> ALAPRQVLDLEDLVFTQGSHFMANKRCQLPDGSFRRQRKGYEEVHVPALKPKPFGSEEQLLPVEKLPKYAQAGFEGFKTLNRIQSKLYRAALETDENLLLCAPTGAGKTNVALMCMLREIGKHINMDGTINVDDFKIIYIAPMRSLVQEMVGSFGKRLATYGITVAELTGDHQLCKEEISATQIIVCTPEKWDIITRKGGERTYT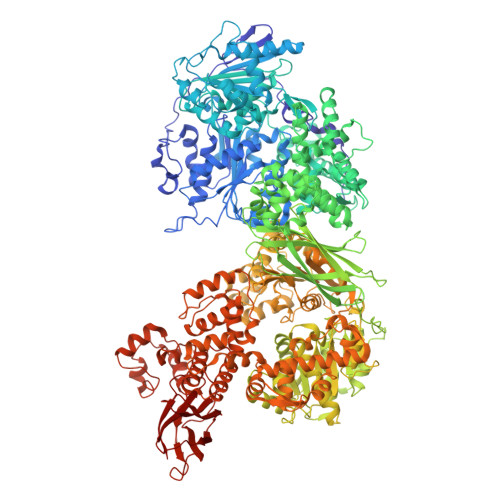QLVRLIILDEIHLLHDDRGPVLEALVARAIRNIEMTQEDVRLIGLSATLPNYEDVATFLRVDPAKGLFYFDNSFRPVPLEQTYVGITEKKAIKRFQIMNEIVYEKIMEHAGKNQVLVFVHSRKETGKTARAIRDMCLEKDTLGLFLREGSASTEVLRTEAEQCKNLELKDLLPYGFAIHHAGMTRVDRTLVEDLFADKHIQVLVSTATLAWGVNLPAHTVIIKGTQVYSPEKGRWTELGALDILQMLGRAGRPQYDTKGEGILITSHGELQYYLSLLNQQLPIESQMVSKLPDMLNAEIVLGNVQNAKDAVNWLGYAYLYIRMLRSPTLYGISHDDLKGDPLLDQRRLDLVHTAALMLDKNNLVKYDKKTGNFQVTELGRIASHYYITNDTVQTYNQLLKPTLSEIELFRVFSLSSEFKNITVREEEKLELQKLLERVPIPVKESIEEPSAKINVLLQAFISQLKLEGFALMADMVYVTQSAGRLMRAIFEIVLNRGWAQLTDKTLNLCKMIDKRMWQSMCPLRQFRKLPEEVVKKIEKKNFPFERLYDLNHNEIGELIRMPKMGKTIHKYVHLFPKLELSVHLQPITRSTLKVELTITPDFQWDEKVHGSSEAFWILVEDVDSEVILHHEYFLLKAKYAQDEHLITFFVPVFEPLPPQYFIRVVSDRWLSCETQLPVSFRHLILPEKYPPPTELLDLQPLPVSALRNSAFESLYQDKFPFFNPIQTQVFNTVYNSDDNVFVGAPTGSGKTICAEFAILRMLLQSSEGRCVYITPMEALAEQVYMDWYEKFQDRLNKKVVLLTGETSTDLKLLGKGNIIISTPEKWDILSRRWKQRKNVQNINLFVVDEVHLIGGENGPVLEVICSRMRYISSQIERPIRIVALSSSLSNAKDVAHWLGCSATSTFNFHPNVRPVPLELHIQGFNISHTQTRLLSMAKPVYHAITKHSPKKPVIVFVPSRKQTRLTAIDILTTCAADIQRQRFLHCTEKDLIPYLEKLSDSTLKETLLNGVGYLHEGLSPMERRLVEQLFSSGAIQVVVASRSLCWGMNVAAHLVIIMDTQYYNGKIHAYVDYPIYDVLQMVGHANRPLQDDEGRCVIMCQGSKKDFFKKFLYEPLPVESHLDHCMHDHFNAEIVTKTIENKQDAVDYLTWTFLYRRMTQNPNYYNLQGISHRHLSDHLSELVEQTLSDLEQSKCISIEDEMDVAPLNLGMIAAYYYINYTTIELFSMSLNAKTKVRGLIEIISNAAEYENIPIRHHEDNLLRQLAQKVPHKLNNPKFNDPHVKTNLLLQAHLSRMQLSAELQSDTEEILSKAIRLIQACVDVLSSNGWLSPALAAMELAQMVTQAMWSKDSYLKQLPHFTSEHIKRCTDKGVESVFDIMEMEDEERNALLQLTDSQIADVARFCNRYPNIELSYEVVDKDSIRSGGPVVVLVQLEREEEVTGPVIAPLFPQKREEGWWVVIGDAKSNSLISIKRLTLQQKAKVKLDFVAPATGAHNYTLYFMSDAYMGCDQEYKFSVD> XKLNLQFFAS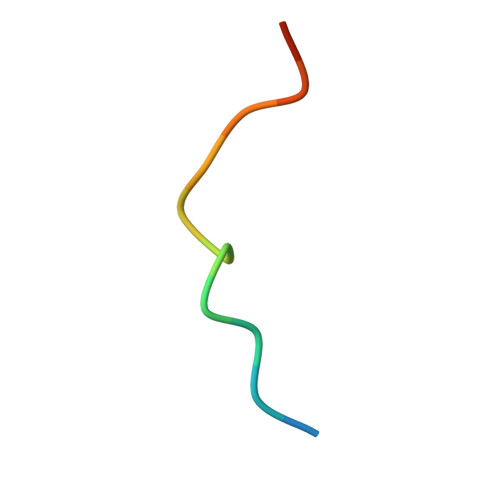KKGX> QGNPNY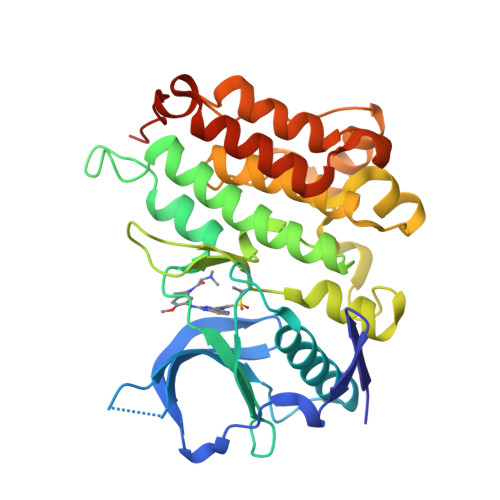CFAGKTSSISDLKEVPRKNITLIRGLGHGAFGEVYEGQVSGMPNDPSPLQVAVKTLPEVCSEQDELDFLMEALIISKFNHQNIVRCIGVSLQSLPRFILLELMAGGDLKSFLRETRPRPSQPSSLAMLDLLHVARDIACGCQYLEENHFIHRDIAARNCLLTCPGPGRVAKIGDFGMARDIYRAGYYRKGGCAMLPVKWMPPEAFMEGIFTSKTDTWSFGVLLWEIFSLGYMPYPSKSNQEVLEFVTSGGRMDPPKNCPGPVYRIMTQCWQHQPEDRPNFAIILERIEYCTQDPDVINTALPIEYGPLVEEEEK> MANQQIGGSTVTYNGAIPMGGPVAINSVIEIAGTEVLVDLKLDY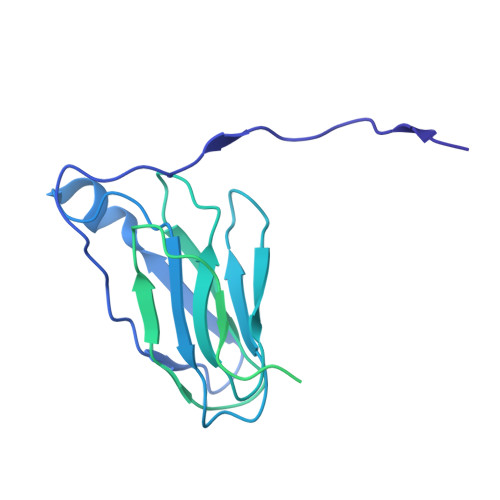ATGKISGVQTLYIDLRDFLGDVTVTMPDTGQRITARAGTQGYYPVLSTNLMKFIVSATIDGKFPMNFINFPIALGVWPSGIKGDKGDPGAPGPAGGTVVVEDSGASFGESLLDTTSEPGKILVKRISGGSGITVTDYGDEVEIEASGGGGGGGGVTDALSLMYSTSTGGPASIAANALTDFDLSGALTVNTVGTGLTKSAAGIQLAAGKSGLYQITMTVKNNTVTTGNYLLRVKYGSSDFVVACPASSLTAGGTISLLIYCDVLGVPSLDVLKFSLCNDGAALSNYIINITAAKIN>[3x]GPTADLGAVIDFSEAHLARSPKPGVPQVVRFPLNVSSVTERDAERVGLEPVSKWRAYGLEGYPGFIFIPNPFLPGCQRHWVKQCLKLYSQKPNVCNLDKHMTKEETQGLWEQSKEVLRSKEVTKRRPRSLLERLRWVTLGYHYNWDSKKYSADHYTPFPSDLAFLSEQVATACGFQGFQAEAGILNYYRLDSTLGIHVDRSELDHSKPLLSFSFGQSAIFLLGGLKRDEAPTAMFMHSGDIMVMSGFSRLLNHAVPRVLPHPDGECLPHCLETPLPAVLPSNSLVEPCSVEDWQVCATYLRTARVNMTVRQVLATGQDFPLEPVEETKRDIAADG

AlkB family of 2-oxoglutarate (2OG or α-KG)-dependent oxygenases are evolutionarily conserved and implicated in nucleotide demethylation. Mouse ALKBH1 protein has 389 residues and consists of an N-terminal extension (NTE), a nucleotide-recognition lid (NRL), and a C-terminal double-stranded β helix (DSBH) domain. By establishing a reliable in vitro enzymatic assay, we demonstrated that ALKBH1 prefers bubbled and bulged DNAs, instead of ssDNA or dsDNA substrates. Structural studies of ALKBH1 in substrate-free and a 21-mer bulge DNA-bound state revealed the molecular determinants underlying the observed substrate preference, including unique features of a stretch-out Flip1 motif and a functionally indispensable N-terminal “α1” helix.

The extra α1 helix forms extensive hydrophobic contacts with the minor sheet involving residues F23, L26, F27, Y30 of α1, I230 of β(II), P290 of β(VII), and I253, L255 of β(IV), and sequence alignment shows that these residues are highly conserved in vertebrates. The α1 helix is critical to maintain the structural integrity of the active center; in particular, F23 and F27 directly stabilize the minor β sheet through extensive hydrophobic contacts. In support, the structure of an N-truncated ALKBH1 (residue 37–369, ALKBH1Δα1) determined at 2.3 Å by the Se-SAD method demonstrates that missing of α1 helix (residues 22–32) results in distortion of the co-factor coordination geometry as reflected by flipping away of H287 and disordering of β(II) that comprises H231 and D233. Neither Mn(II) nor NOG was observed in the crystal, and the impaired co-factor coordination of ALKBH1Δα1 in solution was also confirmed by calorimetric titration. Furthermore, enzymatic assays showed that ALKBH1Δα1 was totally inactive in N6-mA demethylation. Although an α1-truncated human ALKBH1 protein was reported to have demethylation activities towards m1rA in tRNA,8 we performed in vitro enzymatic assay using the α1-truncated human ALKBH1 and hardly detected any activities towards m1rA in tRNA stem loop nor N6-mA in DNA bubble, further underlying the importance of α1 helix.>[4x]MAELACFCYPHLENDSYKFIPFNNLAIKAMLTAKVDKKDMDKFYDSIIYGIAPPPQFKKRYNTNDNSRGMNFETIMFTKVAMLICEALNSLKVTQANVSNVLSRVVSIRHLENLVIRKENPQDILFHSKDLLLKSTLIAIGQSKEIETTITAEGGEIVFQNAAFTMWKLTYLEHQLMPILDQNFIEYKVTLNEDKPISDVHVKEL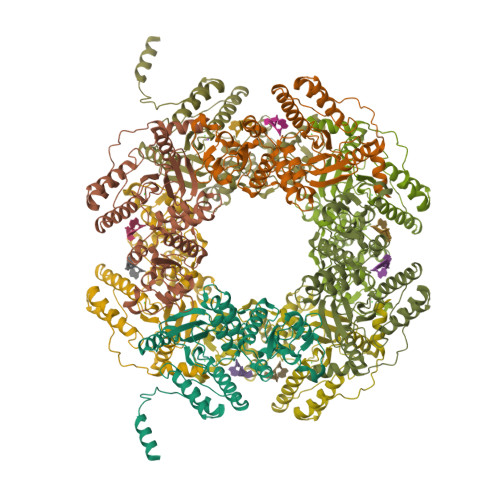VAELRWQYNKFAVITHGKGHYRIVKYSSVANHADRVYATFKSNVKTGVNNDFNLLDQRIIWQNWYAFTSSMKQGNTLDVCKRLLFQKMKPEKNPFKGLSTDRKMDEVSQVGV> DEPGVATGNGQPVTGNWLAGASQGDGVPIPSQIADQLRGKEFKSWRDFREQFWVAVANDPELVKYFRKTNAKGMRDGLSPFTPKAEQAGGRDKYAIHHVVQISQGGAVYDIDNLRVMTPKMHIQV;> SKKISDHTEAEFFSLISELFNRSFSSEK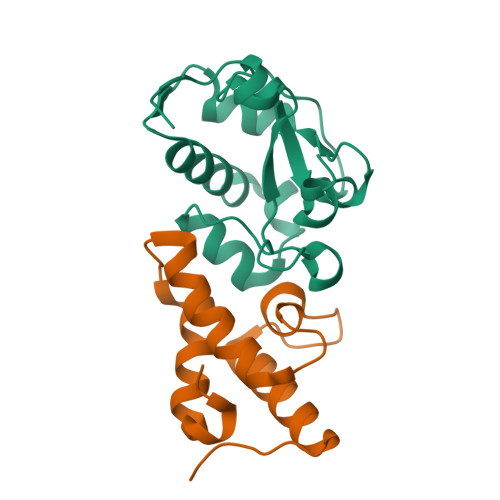ERDVVVYAIVNAAQHPDGTDIIFYPKEDEEDSPEGVLKRIKEWRAANGLPGFKA Typically, the type IV pili are helical polymers constituted of one protein component, the major pilin. Type IV pili not only serve as multifunctional organelles allowing the adherence to host cells and the auto-aggregation of these bacteria, but also play an essential role in their pathogeneses. Molecular dynamics of the whole pilus with GATDH and G3P for a period of 1µs showed the overall stability of the structure. As previously described, the PilE monomer contains a 4 strand beta-sheet region, and an N-terminal melted alpha helix that forms the core of the type-IV pilus. Immune evasion against antibodies targeting type IV pili is thus attributed to the structural diversity present among strains, including variations in pilin sequence, sugar type, and phosphoform.

To better understand the structural bases of the variation in type IV pili surface, i.e. PTM and sequence variation, we determined the native structure of type IV pili purified from two N. meningitidis sequence types, SB and SA, of the 8013 strain genetically modified to have reduced antigenic variation. This strain expresses a class I pilin of the SB type, a GATDH sugar on S63 and G3P phosphoform on S69. The final cryo-EM map of pili (left, SB sequence type, GATDH, G3P) at an average 2.9 Å resolution was generated from iterative helical refinements. The density was sufficient to identify the locations and positioning of GATDH (yellow) and glycerol-3-phosphate (G3P, red), as well as for building atomic models of monomers or multimers of PilE. The phosphoglycerol appears clearly on S69 pointing away from the structure. Molecular dynamics simulations suggest that the glycerol portion of the molecule undergoes rotational motion, which is supported by the lower resolution observed in its electron microscopy (EM) density compared to the phosphate atom. Interestingly, the proximity and relative positioning of GATDH to E56 suggests the presence of a hydrogen O − H···:O bond. Accordingly, molecular dynamics shows that the allowed C8-C9-C10 bond rotations in GATDH allows O5 at the tip of the sugar to rotate, which in some cases permits PilE to alternate between one and two simultaneous hydrogen bonds between E56 and the sugar. Analysis of the dynamics of hydrogen bonds formed between GATDH and E56 side chains over a 1µs period shows that they are present 42% of the time (SD = 18%, average of 30 pilin monomers). This further confirms that the GATDH is mostly immobilized with limited rotation, and might furthermore apply to most strains as E56 is highly conserved in pilin sequences.

> FTLIELMIVIAIVGILAAVALPAYQDYTARAQVSEAILLAEGQKSAVTEYYLNHGEWPGDNSSAGVATSADIKGKYVQSVTVANGVITAQMASSNVNNEIKSKKLSLWAKRQNGSVKWFCGQPVTRTTATATDVAAANGKTDDKINTKHLPSTCRDDSSAS> MPQSFTSIARIGDYILKSPVLSKLCVPVANQFINLAGYKKLGLKFDDLIAEENPIMQTALRRL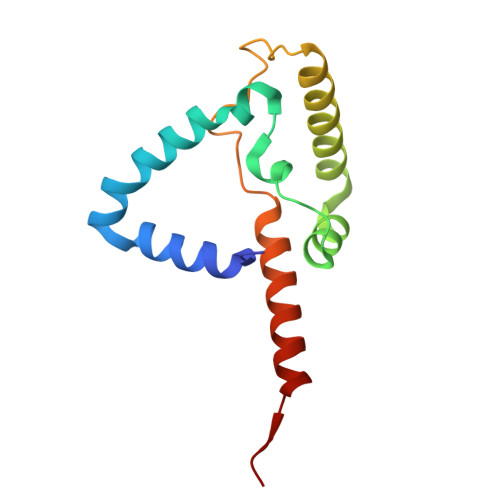PEDESYARAYRIIRAHQTELTHHLLPRNEWIKAQEDVPYLLPYILEAEAAAKEKDELDNIEVSK THIAMINE DIPHOSPHATE | C12 H19 N4 O7 P2 S | 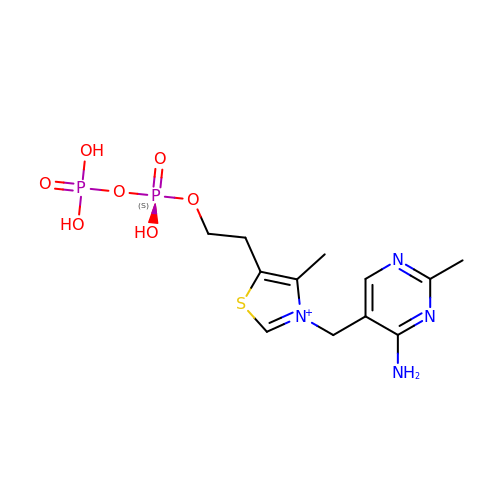AYEKOFBPNLCAJY-UHFFFAOYSA-O> MHHHHHHSSGRENLYFQGIVPRSFRLLDELERGQKGNVSEGVSFGLESADDITLSNWSCTIFGQPGTVFENRIYSLTIFCDDNYPDSPPTVKFDTKIEMSCVDNCGRVIKNNLHILKNWNRNYTIETILI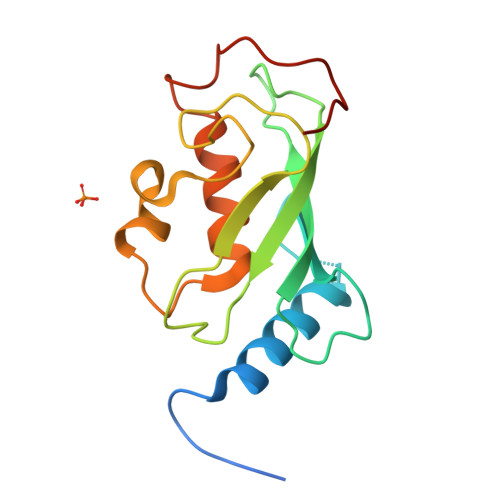SLRQEMLSSANKRLPQPNEGEVYSNN>MKYVVVSGGVISGIGKGVL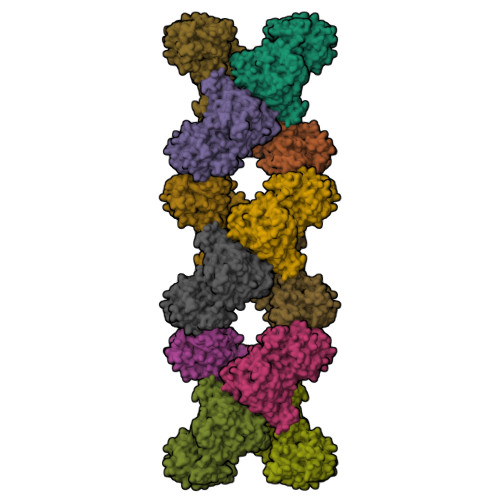ASSTGMLMKTLGLKVTSIKIDPYMNIDAGTMSPLEHGECFVLDDGGETDLDLGNYERYLGVTLTKDHNITTGKIYSHVIAKERKGDYLGKTVQIVPHLTNAIQDWIERVAKIPVDDTGMEPDVCIIELGGTVGDIESAPFVEALRQFQFKVGKENFALIHVSLVPVIHGEQKTKPTQAAIKGLRSLGLVPDMIACRCSETLDKPTIDKIAMFCHVGPEQVVNVHDVNSTYHVPLLLLEQKMIDYLHARLKLDEISLTEEEELLSKWKATTGNFDETVKIALVGKYTNLKDSYLSVIKALEHSSMKCRRKLDIKWVEATDLEPEAQESNKTKFHEAWNMVSTADGILIPGGFGVRGTEGMVLAARWARENHIPFLGVCLGLQIATIEFTRSVLGRKDSHSAEFYPDIDEKNHVVVFMMRLGLRPTFFQNETEWSQIKKLYGDVSEVHERHRHRYEINPKMVDELENNGLIFVGKDDTGKRCEILELKNHPYYIATQYHPEYTSKVLDPSKPFLGLVAASAGILQDVIEGKYDLEA[12x]> ADVTITV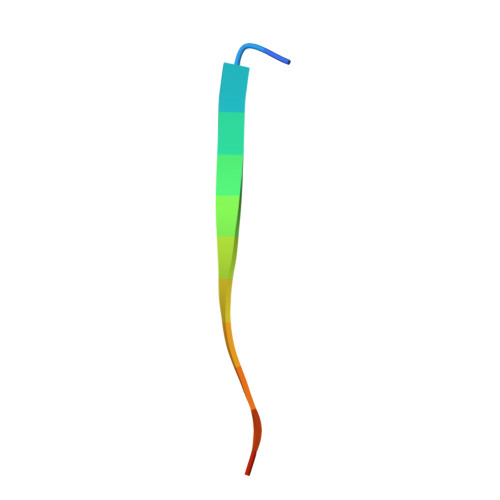NGKVVAK>MTTAGVSRRPGRLAGKAAIVTGAAGGIGRATVEAYLREGASVVAMDLAPRLAATRYEEPGAIPIACDLADRAAIDAAMADAVARLGGLDILVAGGALKGGTGNFLDLSDADWDRYVDVNMTGTFLTCRAGARAMVAAGAGKDGRSARIITIGSVNSFMAEPEAAAYVAAKGGVAMLTRAMAVDLARHGILVNMIAPGPVDVTGNNTGYSEPRLAEQVLDEVALGRPGLPEEVATAAVFLAEDGSSFITGSTITIDG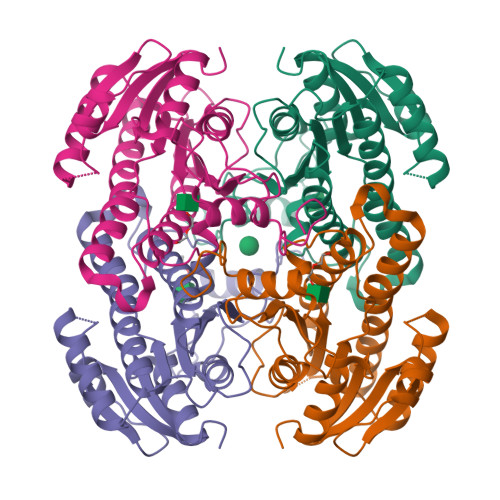GLSAMIFGGMREGRR[16x]>MGIRELNLTKEQHEWLNG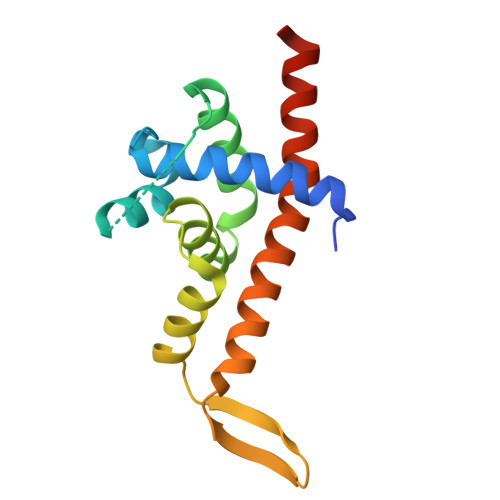WLELWGAWVYSGRLEKRMSSVIAKFMESVEPGRVMTRPMCNDDDGMLISQVVDSVMYIDKKAFGILLSYYAHGSSKHAIASYYHRVARPRKMLCRGGGRIQKPSLATCRREVDEILNASLFMIYPVLDSAFKNRKRVEKIKHVA[2x]> MILLDTNVISEPLRPQPNERVVAWLDSLILEDVYLSAITVAELRLGVALLLNGKKKNVLHERLEQSILPLFAGRIL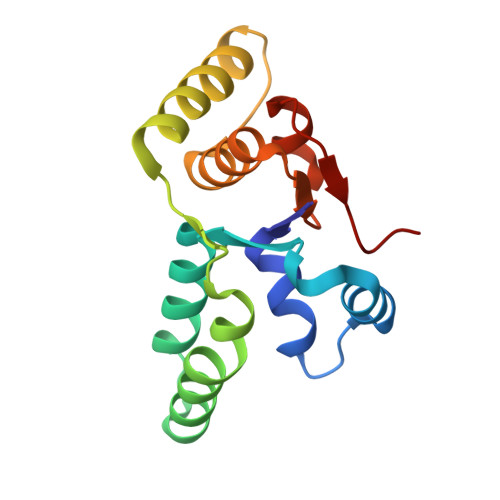PFDEPVAAIYAQIRSYAKTHGKEIAAADGYIAATAKQHSLTVATRDTGSFFAADVAVFNPWHL>[2x]GDITHMAPSRKFFVGGNWKMNGRKQSLGELIGTLNAAKVPADTEVVCAPPTAYIDFARQKLDPKIAVAAQNCYKVTNGAFTGEISPGMIKDCGATWVVLGHSERRHVFGESDEL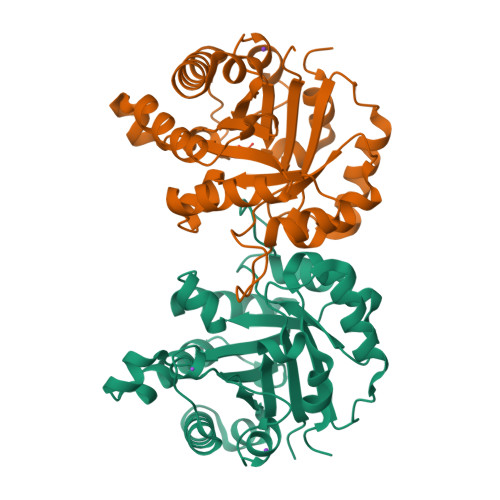IGQKVAHALAEGLGVIACIGEKLDEREAGITEKVVFEQTKVIADNVKDWSKVVLAYEPVWAIGTGKTATPQQAQEVHEKLRGWLKSNVSDAVAQSTRIIYGGSVTGATCKELASQPDVDGFLVGGASLKPEFVDIINAKQ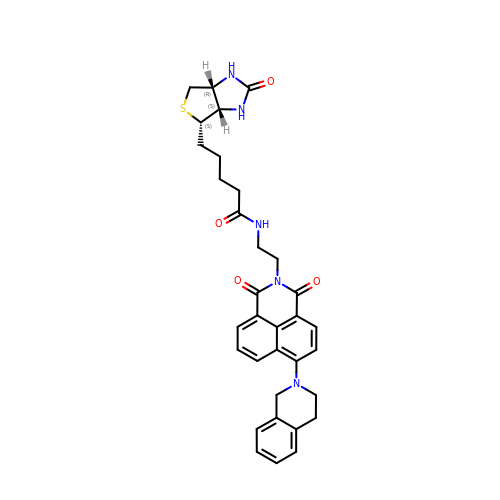5-[(3~{a}~{S},4~{S},6~{a}~{R})-2-oxidanylidene-1,3,3~{a},4,6,6~{a}-hexahydrothieno[3,4-d]imidazol-4-yl]-~{N}-[2-[6-(3,4-dihydro-1~{H}-isoquinolin-2-yl)-1,3-bis(oxidanylidene)benzo[de]isoquinolin-2-yl]ethyl]pentanamide | C33 H35 N5 O4 S | OIYWBNMJMDVZAF-XXJPWZBZSA-N> MTSRDGYQWTPETGLTQGVTSLGVISPPTNIEDTDKDGPWDVIVIGGGYCGLTATRDLTVAGFKTLLLEARDRIGGRSWSSNIDGYPYEMGGTWVHWHQSHVWREITRYKMHNALSP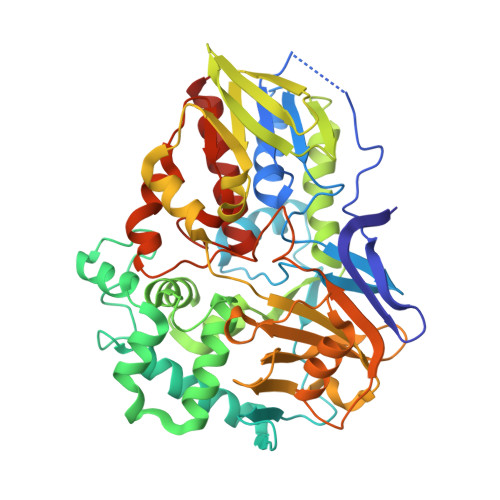SFNFSRGVNHFQLRTNPTTSTYMTHEAEDELLRSALHKFTNVDGTNGRTVLPFPHDMFYVPEFRKYDEMSYSERIDQIRDELSLNERSSLEAFILLCSGGTLENSSFGEFLHWWAMSGYTYQGCMDCLMSYKFKDGQSAFARRFWEEAAGTGRLGYVFGCPVRSVVNERDAARVTARDGREFVAKRVVCTIPLNVLSTIQFSPALSTERISAMQAGHVSMCTKVHAEVDNKDMRSWTGIAYPFNKLCYAIGDGTTPAGNTHLVCFGTDANHIQPDEDVRETLKAVGQLAPGTFGVKRLVFHNWVKDEFAKGAWFFSRPGMVSECLQGLREKHGGVVFANSDWALGWRSFIDGAIEEGTRAARVVLEELGTKREVKARL> VTKPTIAAVGGYAMNNGTGTTLYTKAADTRRSTGSTTKIMTAKVVLAQSNLNLDAKVTIQKAYSDYVVANNASQAHLIVGDKVTVRQLLYGLMLPSGNDAAYALADKYGSGSTRAARVKSFIG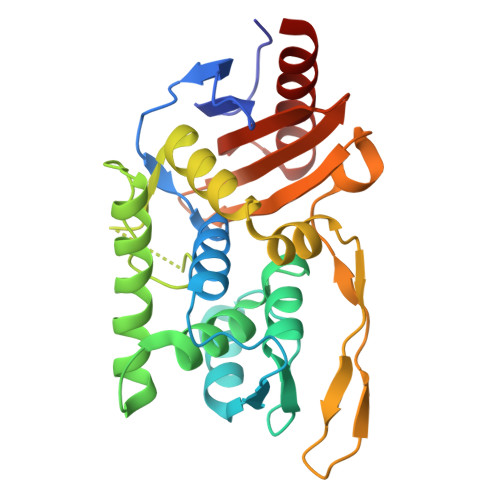KMNTAATNLGLHNTHFDSFDGIGNGANYSTPRDLTKIASSAMKNSTFRTVVKTKAYTAKTVTKTGSIRTMDTWKNTNGLLSSYSGAIGVKTGSGPEAKYCLVFAATRGGKTVIGTVLASTSIPARESDATKIMNYGFAL> KDSSDEASVSPIADNEREAVTLLLGYLEDKDQLDFYSGGPLKALTTLVYSDNLNLQRSAALAFAEITEKYVRQVSREVLEPILILLQSQDPQIQVAACAALGNLAVNNENKLLIVEMGGLEPLINQMMGDNVEVQCNAVGCITNLATRDDNKHKIATSGALIPLTKLAKSKHIRVQRNATGALLNMTHSEENRKELVNAGAVPVLVSLLSSTDPDVQYYCTTALSNIAVDEANRKKLAQTEPRLVSKLVSLMDSPSSRVKCQATLALRNLASDTSYQLEIVRAGGLPHLVKLIQSDSIPLVLASVACIRNISIHPLNEGLIVDAGFLKPLVRLLDYKDSEEIQCHAVSTLRNLAASSEKNRKEFFESGAVEKCKELALDSPV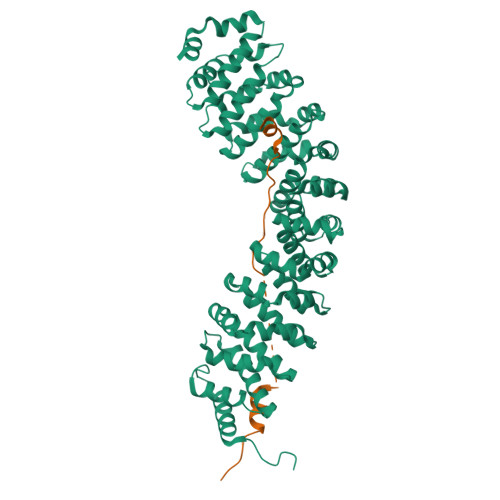SVQSEISACFAILALADVSKLDLLEANILDALIPMTFSQNQEVSGNAAAALANLCSRVNNYTKIIEAWDRPNEGIRGFLIRFLKSDYATFEHIALWTILQLLESHNDKVEDLVKNDDDIINGVRK;> SSASFFRPSNPTFGTSISNVQVNCHPTVAATMAPSRNGPRISSSKALLSSFIARSD> MGLLSDPVRRRALARLVLRLNAPLCVLSYVAGIAWFLALVFPPLTQRTYMSENAMGSTMVEEQFAGGDRARAFARDFAAHRKKSGALPVAWLERTMRSVGLEVYTQSFSRKLPFPDETHERYMVSGTNVYGILRAPRAASTESLVLTVPCGSDSTNSQAVG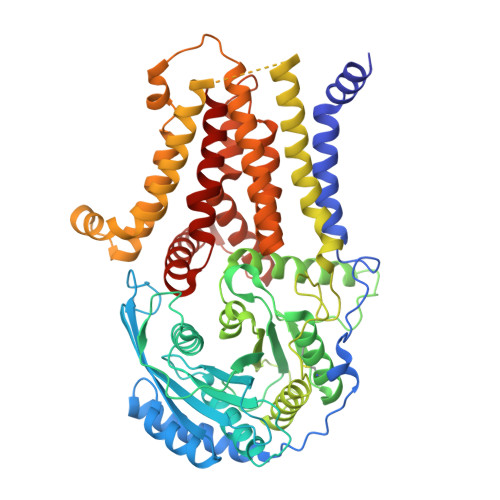LLLALAAHFRGQIYWAKDIVFLVTEHDLLGTEAWLEAYHDVNVTGMQSSPLQGRAGAIQAAVALELSSDVVTSLDVAVEGLNGQLPNLDLLNLFQTFCQKGGLLCTLQGKLQPEDWTSLDGPLQGLQTLLLMVLRQASGRPHGSHGLFLRYRVEALTLRGINSFRQYKYDLVAVGKALEGMFRKLNHLLERLHQSFFLYLLPGLSRFVSIGLYMPAVGFLLLVLGLKALELWMQLHEAGMGLEEPGGAPGPSVPLPPSQGVGLASLVAPLLISQAMGLALYVLPVLGQHVATQHFPVAEAEAVVLTLLAIYAAGLALPHNTHRVVSTQAPDRGWMALKLVALIYLALQLGCIALTNFSLGFLLATTMVPTAALAKPHGPRTLYAALLVLTSPAATLLGSLFLWRELQEAPLSLAEGWQLFLAALAQGVLEHHTYGALLFPLLSLGLYPCWLLFWNVLFWK N-({6-[(4-CYANOBENZYL)OXY]NAPHTHALEN-2-YL}SULFONYL)-D-GLUTAMIC 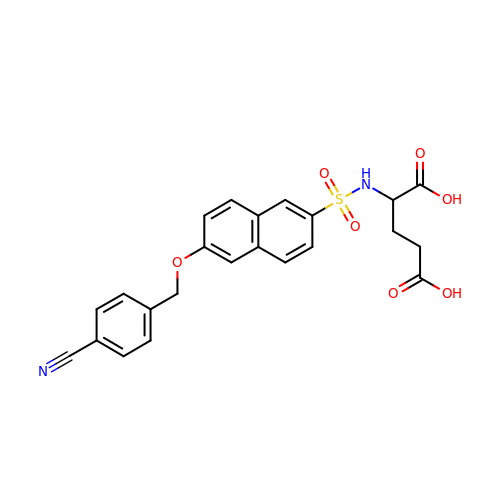ACID | C23 H20 N2 O7 S | PUHRQSFXADUGJW-OAQYLSRUSA-N>MHHHHHHHHHHENLYFQSAMNKIRKTFQYGKHEVTFETGEMARQATGAVVVRMGDTVLLVSVVAKKEAEEGRDFFPLTVNYQEKTYAAGKIPGGYFKREGRPTEKETLTSRLIDRPLRPLFPKGFTNEVQVIATVLSVDSKVPTDIPAILGASAAIGLSGIPFNGSLGAARVGYRGGEYLLNPSLDELKDSALDLVVAGTRDAVLMVESEAQELPESVMLGAVLHGHQAMQVAIQAIAEFIQEAGGAKWEWEPPTVNTALEKWVVEKSEAPLKKAYQIQEKTARQAQIQAIRDQLLADRAAEREGEENAVNEHELAVIFHELERRIVREQILTGQPRIDGRDTKTVRPITVKVGVLPRSHGSALFTRGETQALVVTTLGTERDAQSIDDLDGDRQEEFIFHYNFPPFCVGEVGFMSGPKRREIGHGRLAKRAVVPVVPTLDKFPYVIRVVSEILESNGSSSMASVCGSSLALMDAGVPTKAPVAGIAMGLIKENDKYAVLSDILGDEDHLGDMDFKVAGTSNGVTALQMDIKI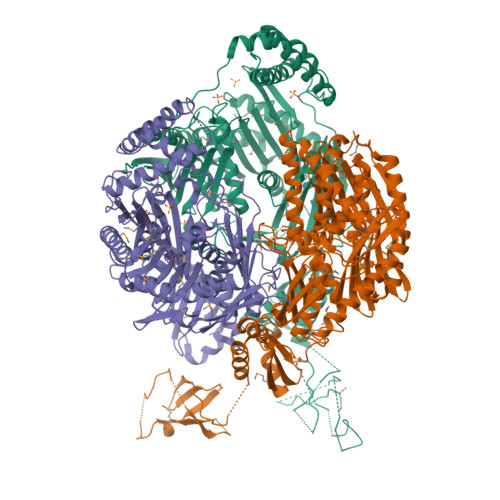EGITKEIMEQALDQAKEGRLHILSIMNKVLDKPRSQVSDLAPQYVTMKINPEKIRDVIGKGGVVIREITEATNCAIDISDDGTIKIAAHTTEEGEAAKRRIEELTAEVELGKVYEGTVVKITDFGAFVQILPNTQGLVHISQIAQERVENVRDYLEEGQVIRVKVIEIDRQGRVRLSMKQID[3x]9-cyclopentyl-N-(5-piperazin-1-ylpyridin-2-yl)pyrido[4,5]pyrrolo[1,2-d]pyrimidin-2-amine 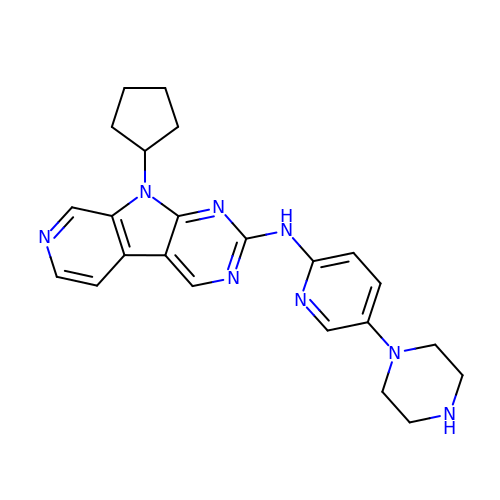| C23 H26 N8 | MCPPMOSBWNMSOA-UHFFFAOYSA-N> GAMGGSEFPKSRLPTLADNEIEYEKQIGKGGFGLVHKGRLVKDKSVVAIKSLILGDSEGETEMIEKFQEFQREVFIMSNLNHPNIVKLYGLMHNPPRMVMEFVPCGDLYHRLLDKAHPIKWSVKLRLMLDIALGIEYMQNQNPPIVHRDLRSPNIFLQSLDENAPVCAKVADFSLSQQSVHSVSGLL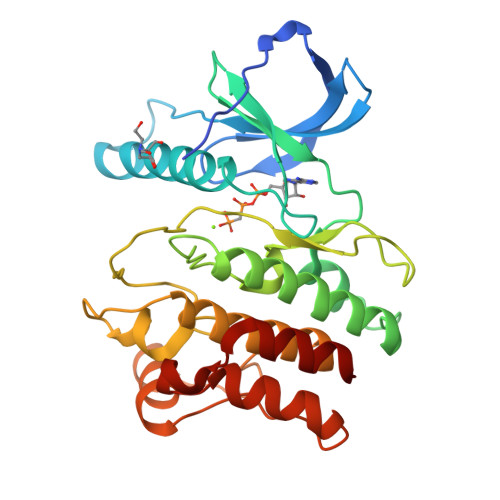GNFQWMAPETIGAEEESYTEKADTYSFAMILYTILTGEGPFDEYSYGKIKFINMIREEGLRPTIPEDCPPRLRNVIELCWSGDPKKRPHFSYIVKELSEL> MARVTVQDAVEKIGNRFDLVLVAARRARQMQVGG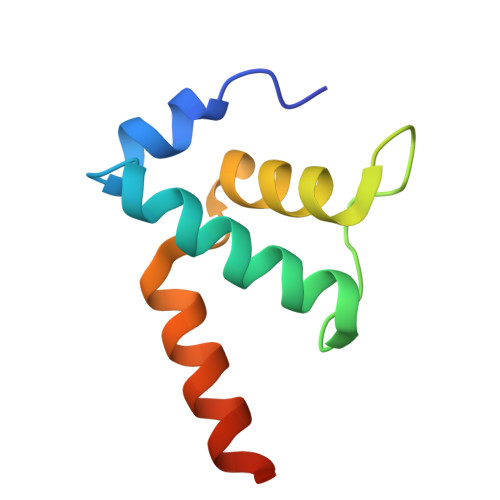KDPLVPEENDKTTVIALREIEEGLINNQILDVRERQEQQEQEAAEL>[6x]MEVICKHYTPLDIASQAIRTCWQSFEY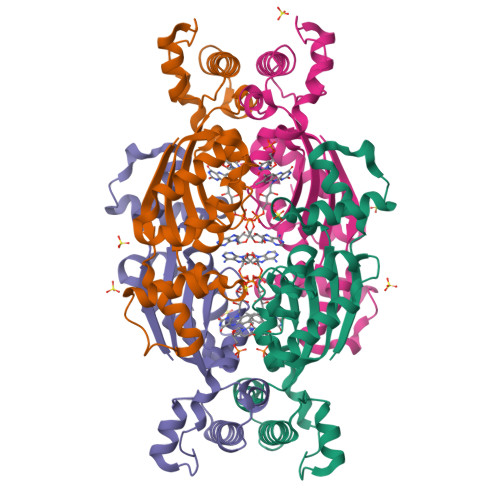SDDGGCKDKELIHRVGNIFRHSSTLEHLYYNFEIKGLSRGALQELSRHRIASLSVKSSRYTLRELKEVESFLPLNETNLERAKEFLVFVDNEKVNAMSVLALENLRILLSEHNIKNDLAKYAMPESYKTHLAYSINARSLQNFLTLRSSNKALKEMQDLAKALFDALPGEHQYLFEDCLKHLEHHHHHH> MKHHHHHHHGAAGTSLYKKAGENLYFQGSMAPRAGFDAEQVRDKARKDLLHLLEGVRGKKNLVIEKDLAGPLGVIVKASTLRDYGVDNFFFLENKNTGTSQRNIVFIARGESVRNAHAIAAQIKRIQRESQTSHDFHIFWVPRRTLFSDKVLEEAGVLGDANISELPLYFFPLERDVLSLELNDSFRDLYLAKDPTPVFLLSRALMGIQKKHGLFPRIIGKGENAKRVADLLSRMRQELLAGEEAGESDRAGLSPSTTIESVIIIDREVDFVTPLLTQLTYEGLIDEYFGIQNNQTDVDAVIVGAPAQSAASTSTAVPTNSSQSRKRKIQLDGSDSLYSQLRDANFAIVGSLLNTVARRLKSDYESRHNTKTTAELKEFVKKLPGYQAEQQSLKIHSNIAEEIINYTRTEIFNKLLEVQQNLAAGADPSSQFDSIEELVARDTPLPQVLRLLCLYSCISGGIKTKELDHFRRLVLQGYGHQHLLTLHNLERLQMFLSKSSPLASMITMSGSSGGPDQKTNYTYLRKQLRLIVDEVNEQDPNDIAYVYSGYAPLSIRLVQCVLQKQYLLSITKGSGTVIAAGPVAGGGAQGWKGFEEIVKHARGPTFDEIQKGEDKAVKARALLSGSSGDKKTVFVVFVGGITFTEIAALRFIAKQEEARRNIVICTTSIINGNRMMNAAIETATFEKTTVTTAAAQ;> MDTAHPTASWEQLGERFYRKIQLYTQVFDQDFDLDNYIVTGAPYGGAIALYRDDEKLVAYQPSRSSRPTIDICSLSGKLLRRISWDQGPIKGVGWSEDEKLLIVMVDGTVRCYFDLQSEFTQFSLGHGAEEHGVKSCRFYSHGLVALLGNNALVSVSSYDEPRPKLLASPPEGRVYSWNIIPPAYSLSRSVEVLLSVNQTIYVCDASECEDRFLDIGPFSHIAVSPNGRFCALYTTTGKVHVITSDFQSRLSEHDTKSKIAPNYFEWCGNDAVVIAWDDEVHLVGPSGSLARFFYDSGRIHLIPDFDGVRILANDRCDFLQKVPDVIEEVFGLGADSPASILLDAVEQLEMKSPKADDNIQLIRPHLVEAVDTCVSAAGQEFSIHWQKQLLKAASFGKSVLDIYNSDDFVDMCETLRVLNAVRFYEVGLPLSYEQYQRLSPSGLISRLLNRHEYLLAIRIADHLRLPTDKIHVHWASAKVRLGSEDDDTICRKIVEKLSGKPGISFEVIARTAYEEGRTRLATELLNHEPRAGRQVPLLLSMEEDELALDKAIESGDTDLIYFVIHQLRRKLPLASFFRVVSSRPTASAMVEALARNSDGDGNEDTALLKDLYYQDDRRLDGASVFIREALQQPETRTASDKLDLAANLLQGNQKEHVFELGALKEAKMLLRMQETFERDLTDSFVGLSVNQTMFKLIKLGYHGRAKKIQSEFKVPERVAWWIRLQALVAKRDWNEIEEISRQRKSPIGWEPFFNQVLQAGNPRLAATFIPKCTNLEPGQTITMYEKCGMRVKAAEEAVRLKDTEAWNRLLEAAGRNTAEGREIERLGATVFKK;> MALDLSSGFAAADAIANLQLADATLPIFEVLPVQLQFSVAADFVAGQAANNVLVIALSNGRILRIDLNKPEDIDDIDLPKKPSEVGVIRRMFLDPTASHLIICTSLGENYYLHSQSRQPRPLARLRGVVIESIAWSPALPTQSTREILIGAADGNIYEAYIETSTEFYRR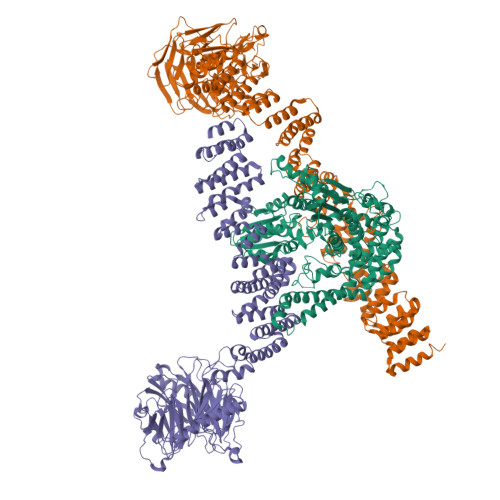EDKYLKLVQKLPDGPITGLWADSLPGHKDTRRVLVATSSRLFHWVGKIGRGHDSGGGASIYDKLFEAEQPTVHALSGASAAAMSMLVVSPDAEQPSPRFREDEVPERAFAWLSSHGVYHGKLLLKGPLSELGAKVFAEAKLLPRAQLANPEGASRRQLSTEYVDAVALTQWHIVSLVAGRVVIANRLTGSIIYDQTILNPGQKAVGLCVDQQKSTFWLFTPQEIFEIVPRDEDRDIWKIMLQLQQFDAALQYAHTPAEKDAVAIASGDHLVSKGQFLEAAAVYGKSSKPFEEVALTFIDNEQPDALRKYLLTKLGTYKKSAVMQRVMIATWLIEVFMAKLNSLDDTIITGAELSETLNPNQTKEQLEAVRAEFQDFINKHKGDLDRKTVYDVIGSHGREEELLYYANAINDYNYVLSYWVQRERWTEALKVLKKQTDPEVFYRYSSVLMTHAATELVEILMRQSNLNPRNLIPAMLEYDRNYKGPLAQNQAVRYLLYVVNQLGSTDSAVHNTLVSIYASHPSKDESALLEYLESQGEEPNYDPDFALRLCIQHRRVLSCAHIYTSMGQYGAAVDLALAHDEVELASIIADRPISNPQLRKKLWLKVAKKVISQQSDGIKTAIDFLRRCDLLKIEDLIPFFPDFVVIDDFKEEICAALEDYSRNIDALRREMDEASQTAANIKVDIAALDKRYAIVEPGEKCYACGLPLLSRQFFVFPCQHAFHSDCLARRVLEQAPPAKARRIKECQVQISKGLVNGEKREAMIAELDALIASACDYAIRRINEPFIKDDDDKDEWAL> GPLGSEITSLDTENIDEILNNADVALVNFYADWCRFSQMLHPIFEEASDVIKEEFPNENQVVFARVDCDQHSDIAQRYRISKYPTLKLFRNGMMMKREYRGQRSVKALADYIRQQKSDPIQEIRDLAEITTLDRSKRNIIGYFEQKDSDNYRVFERVANILHDDCAFLSAFGDVSKPERYSGDNIIYKPPGHSAPDMVYLGAMTNFDVTYNWIQDKCVPLVREITFENGEELTEEGLPFLILFHMKEDTESLEIFQNEVARQLISEKGTINFLHADCDKFRHPLLHIQKTPADCPVIAIDSFRHMYVFGDFKDVLIPGKLKQFVFDLHSGKLHREFHHGPDPTDTAPGEQAQDVASSPPESSFQK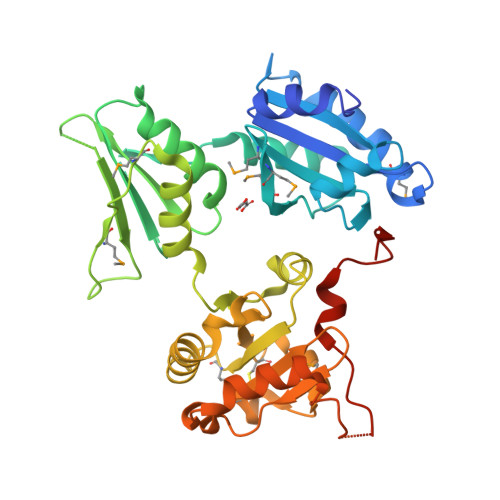LAPSEYRYTLLRDRDEL> MSMNYAAGLSPYADKGKCGLPEIFDPPEELERKVWELARLVWQSSSVVFHTGAGISTASGIPDFRGPHGVWTMEERGLAPKFDTTFESARPTQTHMALVQLERVGLLRFLVSQNVDGLHVRSGFPRDKLAELHGNMFVEECAKCKTQYVRDTVVGTMGLKATGRLCTVAKARGLRACRGELRDTILDWEDS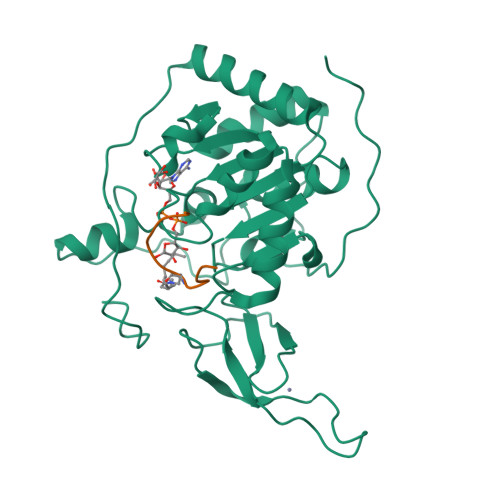LPDRDLALADEASRNADLSITLGTSLQIRPSGNLPLATKRRGGRLVIVNLQPTKHDRHADLRIHGYVDEVMTRLMKHLGLEIPAWDGPRVLERALPPLPRPPTPK;> KQTARXSTGGWW>[2x]AYAQWVIIIIHNVGSKDVKIKNLKPSWGKLHADGDKDTEVSASKYEGTVIKPDEKLQINACGRSDAAEGTTGTFDLVDPADGDKQVRHFYWDCPWGSKTNTWTVSGSNTKWMIEYSGQNLDSGALGTITVDTLKK;> MEAVLSRQAATAEAIGRFQDSSTSVGLVAGSPSTRIRRQADNVVLKSTSQAGDTLNDVIQDPTRRNKLINDNNLLKGIIMGRDGPVPSSRELIVRPDTLRAIINNRATIETTTMEAEFTETLMESNYNSASVKVSAPFITANSEYSESSSFKNTETEKSMYTSSRYLFPQGRIDFT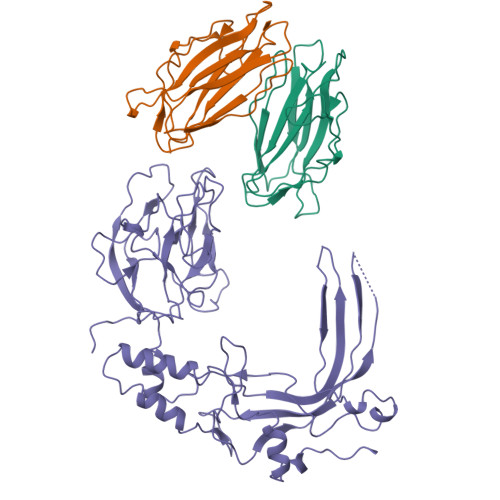TPDSGFDDVIKLSPQFTSGVQAALAKATGTEKREALQNLFQEYGHVFRTKVHIGGVLSAHTMETFSRSENETEVKQDVKAGLEGAVKGWGGGATAGHGNTQGTITTSQNRKLNVKYIVNGGDYTKIQNTEEWVASTNQSEHWRVIEVTEVTAVADLLPQPIRGQVKDLLKPLLGKWVDVEKVPGLESLPVSVYRPKGAIPAGWFWLGDTADASKALLVKPTLPARSGRNPALTSLHQGSGMTEQPFVDLPQYQYLSTYFGSFAHDTPPGSTLRGLRPDHVLPGRYEMHGDTISTAVYVTRPVDVPFPEDECFDLKSLVRVKLPGSGNPPKPRSALKKSMVLFDSGEK NExo is an enzyme from Neisseria meningitidis that is specialized in the removal of the 3′-phosphate and other 3′-lesions, which are potential blocks for DNA repair. NExo is a highly active DNA 3′-phosphatase, and although it is from the class II AP family it lacks AP endonuclease activity. NExo folds into two planes of beta sheets sandwiched between two planes of alpha helices. Notably, the amino acids residues of the active site of the NExo 3′-phosphatase are identical to the active sites of NApe, E. coli Exo III and human APEX1.

To determine the reaction mechanism of the NExo 3′-DNA phosphatase, we solved several crystal structures of NExo with a DNA hairpin substrate containing a 3′-phosphate moiety and a product DNA lacking a 3′-phosphate group. The use of the DNA hairpin structure enabled us to capture the interaction of the enzyme with DNA; we used DNA that forms a short duplex with a 5′ overhang and a phosphate residue at the 3′-end. The structure of the pre-incision substrate DNA complex was solved for wild-type NExo in the absence of metal ions to prevent cleavage. Contacts between the DNA and NExo are mainly through phosphate groups on the DNA backbone, and not via nucleotides; a vast network of indirect interactions is mediated through hydrogen bonding via water molecules. However, our structures of complexes with substrate and product have very similar organization of the active site, either with or without the metal ion cofactor.

> GAMKITTWNVNSLNVRLPQVQNLLADNPPDILVLQELKLDQDKFPAAALQMMGWHCVWSGQKTYNGVAIVSRSVPQDVHFGLPALPDDPQRRVIAATVSGVRVINVYCVNGEALDSPKFKYKEQWFAALTEFVRDEMTRHGKLVLLGDFNIAPADADCYDPEKWHEKIHCSSVERQWFQNLLDLGLTDSLRQVHPEGAFYTWFDYRGAMFQRKLGLRIDHILVSPAMAAALKDVRVDLETRALERPSDHAPVTAEFDW> IVGGQECKDGECPWQALLINEENEGFCGGTILSEFYILTAAHCLYQAKRFKVRVGDRNTEQEEGGEAVHEVEVVIKHNRFTKETYDFDIAVLRLKTPITFRMNVAPACLPERDWAESTLMTQKTGIVSGFGRTHEKGRQSTRLKMLEVPYVDRNSCKLSSSFIITQNMFCAGYDTKQEDACQGDSGGPHVTRFKDTYFVTGIVSWGEGCARKGKYGIYTKVTAFLKWIDRSM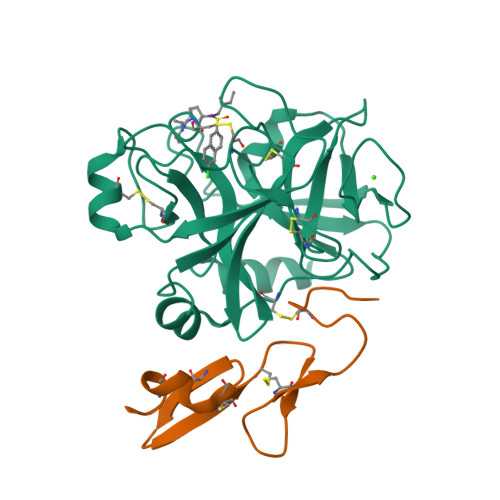KTRGLPKAKSHAPEVITSSPLK;> EEMKKGHLERECMEETCSYEEAREVFEDSDKTNEFWNKYKDGDQCETSPCQNQGKCKDGLGEYTCTCLEGFEGKNCELFTKLCSLDNGDCDQFCHEEQNSVVCSCARGYTLADNGKACIPTGPYPCGKQTLER>MHHHHHHLEVLFQGPLGSEFMLPKYAQVKEEISSWIN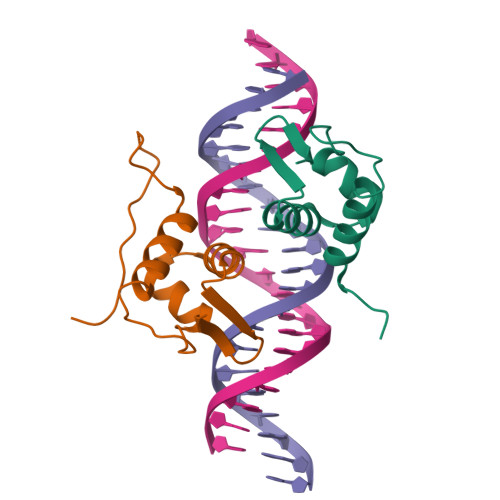QGKILPDQKIPTENELMQQFGVSRHTIRKAIGDLVSQGLLYSVQGGGTFVA[2x]>[2x]MSHLNLDALREVLECPICMESFTEEQLRPKLLHCGHTICRQ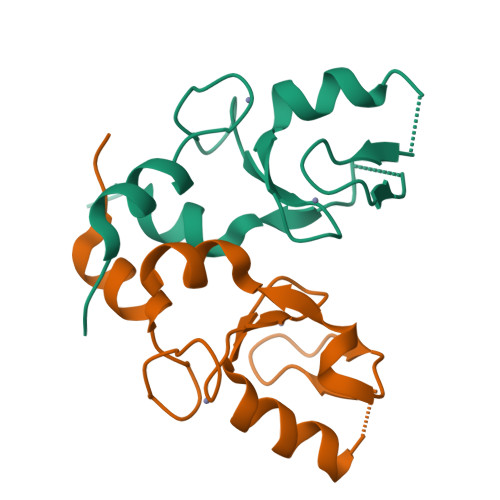CLEKLLASSINGVRCPFCSKITRITSLTQLTDNLTVLKIIDTAGLSEHHHHHH> YNGNPFEGVQLWANNYYRSEVHTLAIPQITDPALRAAASAVAEVPSFQWLDRNVTVDTLLVQTLSEIREANQAGANPQYAAQIVVYDLPDRDCAAAASNGEWAIANNGVNNYKAYINRIREILISFSDVRTILVIEPDSLANMVTNMNVPKCSGAASTYRELTIYALKQLDLPHVAMYMDAGHAGWLGWPANIQPAAELFAKIYEDAGKPRAVRGLATNVANYNAWSVSSPPPYTSPNPNYDEKHYIEAFRPLLEARGFPAQFIV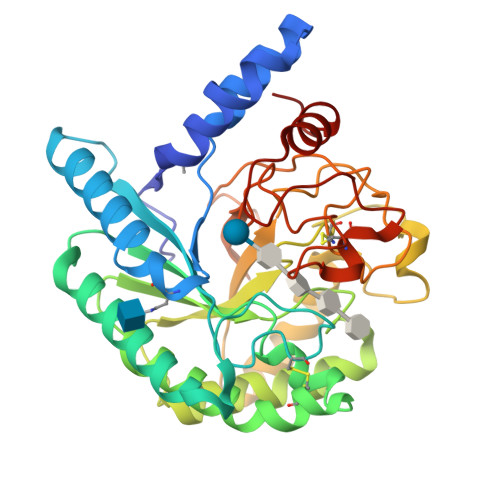DQGRSGKQPTGQKEWGHWCNAIGTGFGMRPTANTGHQYVDAFVWVKPGGECDGTSDTTAARYAYHCGLEDALKPAPEAGQWFNEYFIQLLRNANPPF>NVVTDEPKTDKDVKKLGQDDAGYTIGEE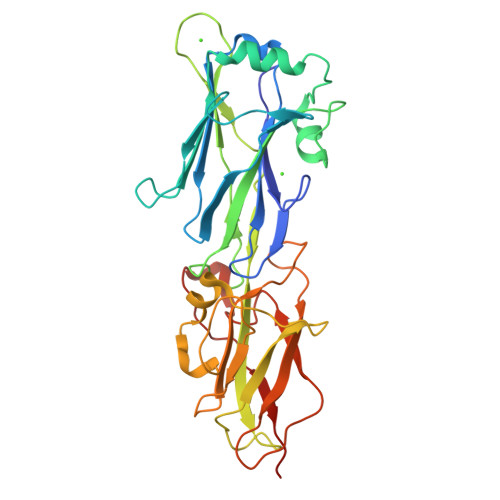FKWFLKSTIPANLGDYEKFEITDKFADGLTYKSVGKIKIGSKTLNRDEHYTIDEPTVDNQNTLKITFKPEKFKEIAELLKGMTLVKNQDALDKATANTDDAAFLEIPVASTINEKAVLGKAIENTFELQYDHTPDKADNPKPSNPPRKPEVHTGGKRFVKKDSTETQTLGGAEFDLLASDGTAVKWTDALIKANTNKNYIAGEAVTGQPIKLKSHTDGTFEIKGLAYAVDANAEGTAVTYKLKETKAPEGYVIPDKEIEFTVSQTSYNTKPTDITVDSADATPDTIKNNKR[2x]> MLNQFPGQYSNNIFCFPPIESETKSGKKASWIICVQVVQHNTIIPITDEMFSTDVKDAVAEIFTKFFVEEGAVRISKMTRVTEGKNLGKKNATTVVHQAFKDALSKYNRHARQKRGAHTNRGMIPPMLVKYFNIIPKTFFEEETDPIVQRKRNGVRAVACQQGDGCILLYSRTEKEFLGLDNIKKELKQLYLFIDVRVYLDGELYLHRKPLQWIAGQANAKTDSSELHFYVFDCFWSDQLQMPSNKRQQLLTNIFKQKEDLTFIHQVENFSVKNVDEALRLKAQFIKEGYEGAIVRNANGPYEPGYNNYHSAHLAKLKPLLDAEFILVDYTQGKKGKDLGAILWVCELPNKKRFVVTPKHLTYADRYALFQKLTPALFKKHLYGKELTVEYAELSPKTGIPLQARAVGFREPINVLEII

AsfvLIG catalyzes the DNA ligation reaction during the base excision repair (BER) process of ASFV genome. AsfvLIG is composed of 419 amino acids and is one of the smallest DNA ligases identified to date. However, unlike the homologous proteins (such as HsLIG1 and SusLIG1), the fidelity of AsfvLIG is very low. By solving four AsfvLIG:DNA complex structures, including the non-catalytic open form and the catalytic closed forms, we showed that the NTD, AD, and OB domains of AsfvLIG undergo a large conformational change during the catalytic assembly.

Our structures represent several different states of the reaction: the AsfvLIG:CG complex structure captured the Watson–Crick C:G pair prior to ligation, whereas AsfvLIG:CT1 and AsfvLIG:CT2 captured the mismatched C:T pair prior to and after the ligation process, respectively. Owing to higher resolution (2.35 Å), the AsfvLIG:CT1 structure was used to demonstrate the overall folding of the catalytic form complexes. Unlike the extended non-catalytic structure, AsfvLIG undergoes large domain rearrangement and adopts a closed conformation in the catalytic AsfvLIG:DNA complex. AsfvLIG is assembled like a ring-shaped clamp and encircles the DNA duplex in its central channel. In the DNA, 19 out of 22 base pairs (bp) is covered by AsfvLIG. The AD domain of AsfvLIG mainly recognizes the broken strand at the nick site and the flanking region upstream, whereas the OB domain primarily interacts with the continuous template strand surrounding and downstream of the nick. As revealed by the AsfvLIG:CT1 structure, the NTD domain forms extensive interactions with the DNA substrate. In the AsfvLIG:CT1 structure, the nucleobases of the template C11 and the nick site T12 form one H-bond (3.1 Å) between their N4 and O4 atoms, respectively. Further, via the water-mediated H-bond, the O2 atom of the C11 nucleobase also interacts with the main chain N atom of Gln403 of the OB domain. Though not identical, the overall shapes and orientations of the C:T pair in AsfvLIG:CT1 and the C:G pair in AsfvLIG:CG are similar.> MTRSRRSGPLDMSTLMGATLGKGKLGYGVQRARALLLWPQAVGPEIARMT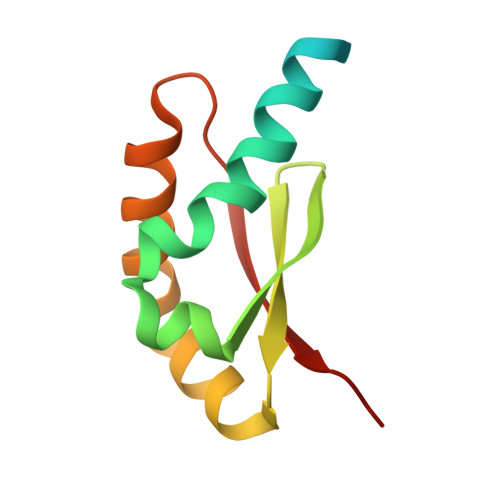RPRSVQGGTLFVEVRDSAAAHHLTMQRHHFLKRLNELLGAGQEVSELRFSVGHIR> QPSFRPSALVVPVKKDASTLQYVTTINQRTPLVSENLVVDLGGRFLWVDCDQNYVSSTYRPVRCRTSQCSLSGSIACGDCFNGPRPGCNNNTCGVFPENPVINTATGGEVAEDVVSVESTDGSSSGRVVTVPRFIFSCAPTSLLQNLASGVVGMAGLGRTRIALPSQFASAFSFKRKFAMCLSGSTSSNSVIIFGNDPYTFLPNIIVSDKTLTYTPLLTNPVSTSATSTQGEPSVEYFIGVKSIKINSKIVALNTSLLSISSAGLGGTKISTINPYTVLETSIYKAVTEAFIKESAARNITRVASVAPFGACFSTDNILSTRLGPSVPSIDLVLQSESVVWTITGSNSMVYINDNVVCLGVV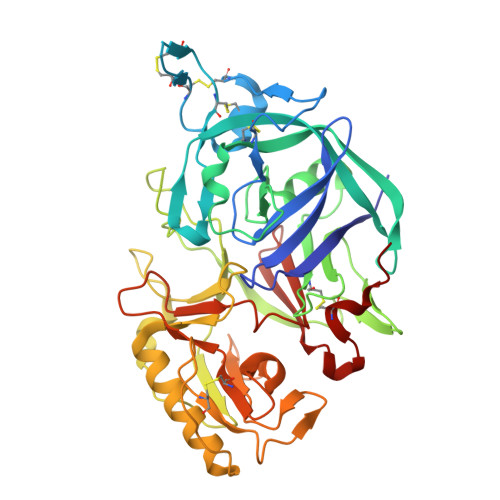DGGSNLRTSIVIGGHQLEDNLVQFDLATSRVGFSGTLLGSRTTCANFNFTS>[2x]MSYASLSVKDLTSLVSRSGTGSSSSLKPPGQTRPVKVIPLQHPDTSNEARPPSIPFDDIFSGWTAKIKRMRLVDWIDTLFPCFRWIRTYRWSEYFKLDLMAGITVGIMLVPQAMSYAKLAGLPPIYGLYSSFVPVFVYAIFGSSRQLAIGPVALVSLLVSNALGGIADTNEELHIELAILLALLVGILECIMGLLRLGWLIRFISHSVISGFTSASAIVIGLSQIKYFLGYSIARSSKIVPIVESIIAGADKFQWPPFVMGSLILVILQVMKHVGKAKKELQFLRAAAPLTGIVLGTTIAKVFHPPSISLVGEIPQGLPTFSFPRSFDHAKTLLPTSALITGV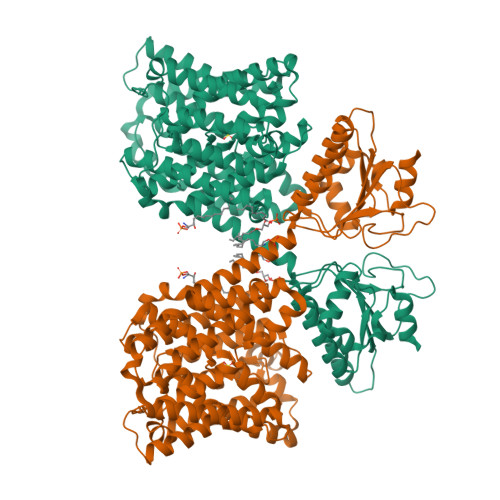AILESVGIAKALAAKNRYELDSNSELFGLGVANILGSLFSAYPATGSFSRSAVNNESEAKTGLSGLITGIIIGCSLLFLTPMFKYIPQCALAAIVISAVSGLVDYDEAIFLWRVDKRDFSLWTITSTITLFFGIEIGVLVGVGFSLAFVIHESANPHIAVLGRLPGTTVYRNIKQYPEAYTYNGIVIVRIDSPIYFANISYIKDRLREYEVAVDKYTNRGLEVDRINFVILEMSPVTHIDSSAVEALKELYQEYKTRDIQLAISNPNKDVHLTIARSGMVELVGKEWFFVRVHDAVQVCLQYVQSSNLEDKHLSFTRRYGGSNNNSSSSNALLKEPLLSVEK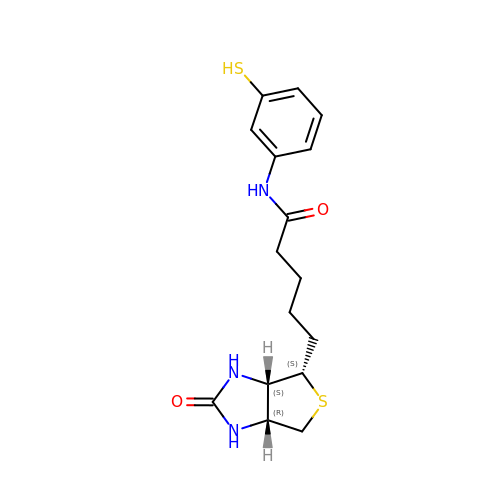5-[(3~{a}~{S},4~{S},6~{a}~{R})-2-oxidanylidene-1,3,3~{a},4,6,6~{a}-hexahydrothieno[3,4-d]imidazol-4-yl]-~{N}-(3-sulfanylphenyl)pentanamide | C16 H21 N3 O2 S2 | HLZRUWZNECQSHZ-YDHLFZDLSA-N>[6x]MKIADIQVRTEHFPLTRPYRIAFRSIEEIDNLIVEIR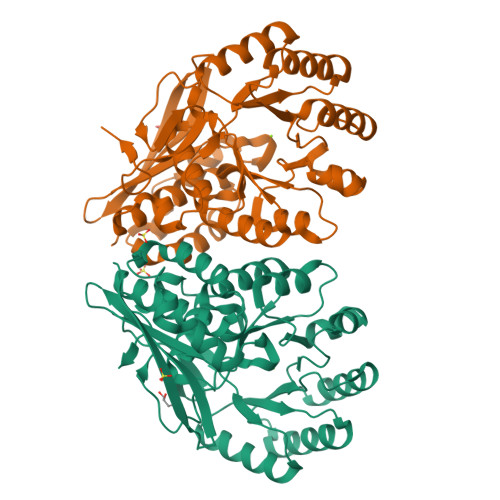TADGLLGLGAASPERHVTGETLEACHAALDHDRLGWLMGRDIRTLPRLCRELAERLPAAPAARAALDMALHDLVAQCLGLPLVEILGRAHDSLPTSVTIGIKPVEETLAEAREHLALGFRVLKVKLCGDEEQDFERLRRLHETLAGRAVVRVDPNQSYDRDGLLRLDRLVQELGIEFIEQPFPAGRTDWLRALPKAIRRRIAADESLLGPADAFALAAPPAACGIFNIKLMKCGGLAPARRIATIAETAGIDLMWGCMDESRISIAAALHAALACPATRYLDLDGSFDLARDVAEGGFILEDGRLRVTERPGLGLVYPD While mammals use G protein-coupled receptors (GPCRs) for sweet and bitter tastant perception, insects such as fruit flies use a unique family of proteins called gustatory receptors (Grs). To unravel the overall structure of these receptors and their unique structure features that define sugar specificity, we determined the cryo-electron microscopy (cryo-EM) structures of Drosophila mojavensis Gr43a (DmoGr43a) (given its better biochemical behavior than Drosophila melanogaster Gr43a (DmGr43a)) and Drosophila melanogaster Gr64a (DmGr64a) in apo or sugar-bound states. As expected, both DmoGr43a and DmGr64a form tetramer, and are topologically similar to each other, and to Orco from Apocrypta bakeri and odorant receptor 5 from Machilis hrabei (MhOR5)11. The structures of DmoGr43a and DmGr64a can be separated into a TMD with 28 transmembranes (TMs) in total (7 TMs in each subunit, numbered as S1–S7), and an intracellular domain (ICD) containing an “anchor domain”, following the nomenclature of Orco/MhOR510,11.

Among different sugars tested, e.g., 100 mM maltose, arabinose, glucose, trehalose, and fructose, only fructose activated DmoGr43a, with a measured EC50 of 42.97 ± 4.69 mM and ~30 mM in electrophysiology and calcium imaging respectively. Fructose, a pentose, adopts a conformation that its five-membered ring is roughly perpendicular to the membrane surface in the fructose-bound DmoGr43a structure. Accurate modeling of bound fructose in DmoGr43a was confirmed using molecular dynamic (MD) simulations, where fructose molecules remained stable. When glucose was placed in the densities, they also have a high probability of stable binding in the pocket according to the MD simulations, in line with the observation that glucose could bind but not activate BmGr9. Binding of fructose in DmoGr43a is achieved by formation of hydrogen bonds and hydrophobic interactions between residues in the binding pocket and various groups of fructose. Notably, Arg 70 from the S1–S2 loop, which is disordered in the apo state, becomes well-resolved in the fructose-bound state, and travels downward for fructose binding. Residues participating in fructose binding are generally very sensitive to mutagenesis, as most mutations rendered the channel non-responsive to fructose at up to 300 mM concentration. In DmoGr43a, Phe 313 from S5, which is directly involved in fructose binding, moves ~1.6 Å towards fructose, together with the whole S5. When the protomer structures of sugar-bound DmoGr43a and DmGr64a were aligned, it shows that these two sugar molecules do not overlap with each other, with the bound fructose molecules positioned closer to the pore in DmoGr43a, and the bound sucrose molecules in DmGr64a positioned further away from the pore. Therefore, sugar-bound structure of DmoGr43a and DmGr64a are likely in desensitized or pre-open states.

>[4x]MEISETNIGIFYVSKLLALAPYSAKKNSKGQLEITRSWLFSIYSVCLCLIMVFLTYRGLLFDANSNIPVRMKSATSKVVTASDVSVVVLAIVTGVYCGMFGLRATQELNTRLDKIDSTLSPYNNVKKDRWRAYAMATVSLIVIGILLGLDVGTWVRMAQEMNISDEDTELNVQWYIPFYSLYFILTGLHINFANTAYGLGRRYKRLNQMLRTSYLSADKSYGNATNLVKVSTVKSISFKPMMPMALHASLTKLNTETLPNESATKNKSLLIRAMADNHESLGKCVRLLSRFYGIAVLFILVSCLLHLVATAYFLFLEMLNKRDNGYVWVQMLWIIFHFLRLLMVVEPCHLAAREARKTIQIVCEIERKVFEPILVEETKKFWQQLLVDDAEFSASGLCRVNRTILTSFASAIATYLVILIQFQKTNGLEGGSSGGWSHPQFEK The capsular polysaccharides (CPSs) surrounding the A. baumannii cells are the primary receptors for bacteriophages encoding specific structural depolymerases that determine the initial step of phage–host interaction. The genomes of Friunaviruses encode only one tailspike depolymerase (TSD) specific to a certain K type or several K types with similar structures or linkages between K units. In the obtained trimeric structures of the TSDs APK09_gp48, APK14_gp49, and APK16_gp47, each chain contains a particle-binding N-terminal domain and a central β-helix domain, as well as a C-terminal domain forming CPS-recognizing/degrading parts. All depolymerases studied were specific glycosidases that cleaved the corresponding CPSs by the hydrolytic mechanism with the production of monomers or/and oligomers (dimers and trimers) of the repeating K units.

In the case of APK16_gp47, the protein includes a part of N-terminal particle-binding domain (residues 154–213), which has three antiparallel β-strands, the following N-terminal helix-turn-helix domain (214–252), a large central right-handed β-helix domain (253–661) having 15 rungs, as well as a C-terminal seven-stranded β-sandwich domain (662–785). Rungs 7–9 (numbering starts from N-terminus) of the β-helix domain are complete rungs and are formed by three β-strands B1, B2, and B3, separated by turns T1, T2, and T3, where B1, B3, and T3 are solvent-exposed, and T2 faces the three-fold symmetry axis of the trimer. Besides β-sheet hydrogen bonding, the β-helix domain is additionally fastened by 18 salt bridges and hydrophobic interactions between inward-facing stacks of side chains of valine, leucine, isoleucine, and phenylalanine. Noteworthy, none of the pairs of stacked cysteines C348, C381, C413, and C434 form disulfide bonds, in spite of their location proximity. APK16_gp47 crystallographic trimer has a diameter of 75Å and a length of about 150Å (without N-terminal particle-binding domain). Each subunit of the trimer has an interface area of about 4928Å2 (16% of the total subunit area). The trimer is stabilized by a total of 201 hydrogen bonds, 27 salt bridges and hydrophobic interactions, mainly between the β-helix domains of three subunits (formed by the side chains of L226, F253, I259, V279, I591, I614, I621, I643, and V650) and between the β-sandwich domain of three subunits (formed by the side chains of I689, I708, L722, L724, I728, V741, I746, and V748). The trimer has two cavities—a small one in the N-terminal domain and a large protruding cavity in the central β-helix domains, which, however, lack solvent molecules. CPS-recognizing/degrading part of APK16_gp47 has no homologs among phage proteins deposited in GenBank but shares amino acid similarity with hypothetical protein (WP_228157370) encoded in A. baumannii genome. Treatment of the CPS with depolymerase APK16_gp47 resulted only in monomer of the K unit.

> GSEVAAAQTQYYLKYFNPDIVYPKNARIMLDTGVVVMSMVDGNSTNPNSNMTGWVRVNSASLIFDQSGKTQQEINDSQKQKLPSLKDYGAVSGQDSTAAIKAAIAAEDFLYFGDIGDNFIVSEQIDLRDGCYYVSNGAKFTAALGIEGSQPYTPKSIINASGKVGINISGLVRTHIDHNIFSALGDANSKPTISGFLADAAIDCDFGKWESVGSVNYYYTPNFKEYGIVDLRNSIDCYIEADVNGRWTEETTASTPSTVGIMGSNNKGCYLKGRAKNCYWSGILWEGEDCVVDGPHVRNTKGSNLNLAGKNTAAYNVDLYGSEQGNISIGEGATQAENCNVVGGVAGNAKFANCHLHSVTKNCHVKLFHYGWGQTASAVSDATSGIRCQGTGNTIDSEFDVTYGGLTVKGDAVNVYCSTLTNPEATNIKVNVVGIGARVQIRAPYTIVNAKITGATGDAVVLGERCKGSIVEEVTAIKCGRPLQYAPKTTDANDYAGVIIGRINDVECTNRSVFYGQKIVHSQRKIERIYAQETAFVLDQVLEAIEVYTNDSGVTGANKLASAIRHISADSFGTSYGLDLVASTISKNNLANSKTKVRAGHIEVEPAVAGAASHIVLYAANGTKWKLEPTGSASAANWVAV P2X receptors (P2XRs) are trimeric, nonselective cation channels activated by adenosine triphosphate (ATP) that act as molecular sensors for extracellular ATP (eATP) (1–8). Predominantly expressed in immune cells, homomeric P2X7 receptors are molecular sensors for pathological inflammatory states by detecting and responding to mid-micromolar to low-millimolar local concentrations of eATP. P2X7 activation triggers signaling cascades that result in up-regulation of the NLRP3 (NOD-, LRR-, and pyrin domain–containing protein 3) inflammasome and activation of apoptotic pathways. Here, we report high-resolution cryo–electron microscopy structures of the homomeric rat P2X7 receptor bound to five previously known small-molecule allosteric antagonists and a sixth antagonist that we identify.

Shallow binders, represented by A438079, A839977, AZD9056, and GSK1482160, extend minimally into the classical allosteric ligand-binding site. The adamantane-containing ligand AZD9056 is also coordinated by hydrophobic interactions and two hydrogen bonds with D92 and Y298, but not with K297. This, together with the increased hydrophobicity of AZD9056, could possibly explain its modest inhibitory potency (IC50 = 330 ± 100 nM). F103 only participates in hydrophobic interactions with AZD9056, GSK1482160, and JNJ47965567. K110 forms cation-pi interactions with A839977 and AZD9056 and hydrogen bonds with GSK1482160 (distance of 2.9 Å). Following a 40-s exposure to an IC100 of antagonist, channel activity recovered more with exposure to AZD9056 and A438079 (82 ± 5% and 81 ± 5% of baseline current, respectively) when compared with exposure to A839977 and GSK1482160 (67 ± 6% and 69 ± 4% of baseline current, respectively). While A438079, AZD9056, and GSK1482160 demonstrated progressively less recovery after longer IC100 exposure times, none of these antagonists completely prevented channel recovery. All shallow binding ligands are too far apart from their symmetrically located counterparts to participate in inter-ligand interactions.

>[3x]MPACCSWNDVFQYETNKVTRIQSVNYGTIKWILHMTVFSYVSFALMSDKLYQRKEPLISSVHTKVKGVAEVTENVTEGGVTKLVHGIFDTADYTLPLQGNSFFVMTNYLKSEGQEQKLCPEYPSRGKQCHSDQGCIKGWMDPQSKGIQTGRCIPYDQKRKTCEIFAWCPAEEGKEAPRPALLRSAENFTVLIKNNIDFPGHNYTTRNILPGMNISCTFHKTWNPQCPIFRLGDIFQEIGENFTEVAVQGGIMGIEIYWDCNLDSWSHRCQPKYSFRRLDDKYTNESLFPGYNFRYAKYYKENGMEKRTLIKAFGVRFDILVFGTGGKFDIIQLVVYIGSTLSYFGLATVCIDLIINTYASTCCRSRVYPSCKCCEPCAVNEYYYRKKCEPIVEPKPTLKYVSFVDEPHIWMVDQQLLGKSLQDVKGQEVPRPQTDFLELSRLSLSLHHSPPIPGQPEEMQLLQIEAVPRSRDSPDWCQCGNCLPSQLPENRRALEELCCRRKPGQCITTSELFSKIVLSREALQLLLLYQEPLLALEGEAINSKLRHCAYRSYATWRFVSQDMADFAILPSCCRWKIRKEFPKTQGQYSGFKYPY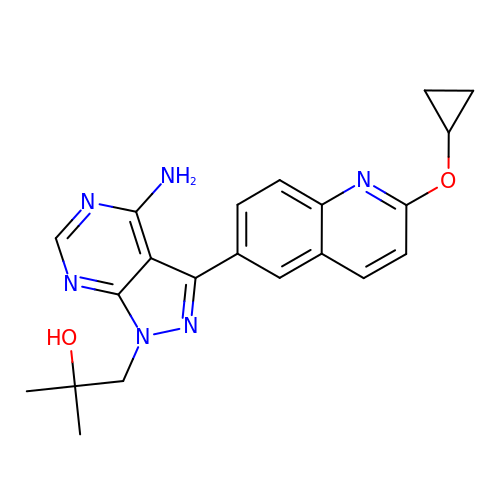1-{4-amino-3-[2-(cyclopropyloxy)quinolin-6-yl]-1H-pyrazolo[3,4-d]pyrimidin-1-yl}-2-methylpropan-2-ol | C21 H22 N6 O2 | NJEBVFDXJAFAGB-UHFFFAOYSA-N> GPLGSEPRSLTAEEVKRLEEQEEDTFRELRIFLRNVTHRLAIDKRFRVFTKPVDPDEVPDYVTVIKQPMDLSSVISKIDLHKYLTVKDYLRDIDLICSNALEYNPDRDPGDRLIRHRACALRDTAYAIIKEELDEDFEQ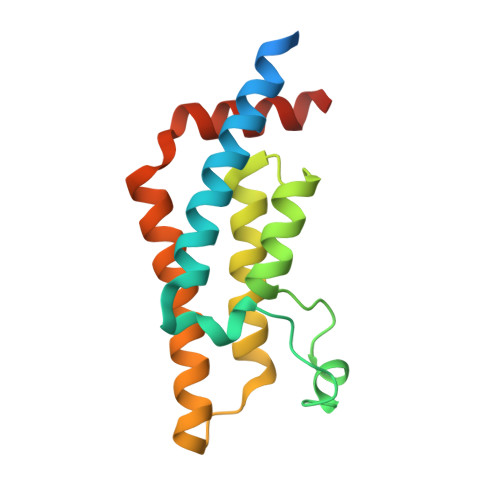LAEEIQESRKKRG> IVGGYTCGANTVPYQVSLNSGYHFCGGSLINSQWVVSAAHCYKSGIQVRLGEDNINVVEGNEQFISASKSIVHPSYNSNTLNNDIMLIKLKSAASLNSRVASISLPTSCASAGTQCLISGWGN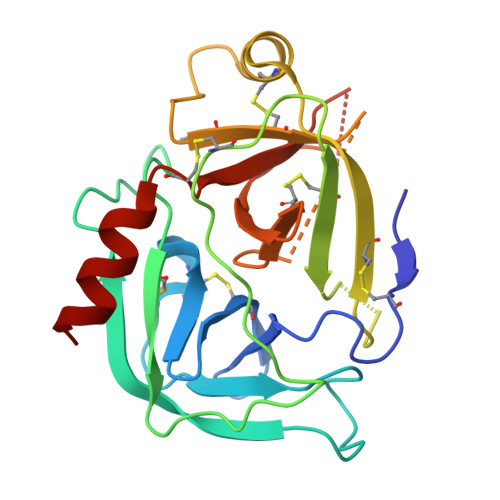TKSSGTSYPDVLKCLKAPILSDSSCKSAYPGQITSNMFCAGYLEGGKDSCQGDAGGPVVCSGKLQGIVSWGSGCAQKNKPGVYTKVCNYVSWIKQTIASN> ER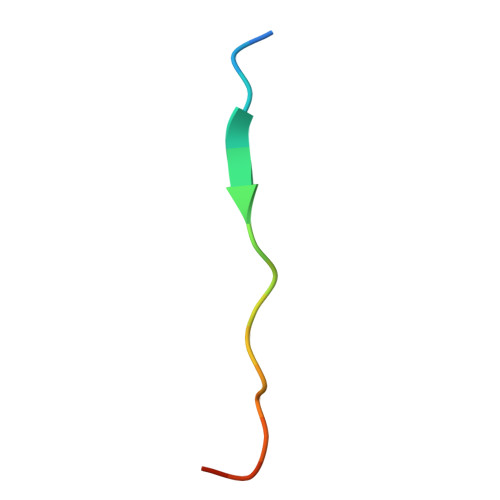ALLFTKPPSDLSAYAD N-(3-azanylpropyl)-3-[[(3S)-1-(2-fluorophenyl)-2-oxidanylidene-pyrrolidin-3-yl]amino]-N-methyl-benzamide 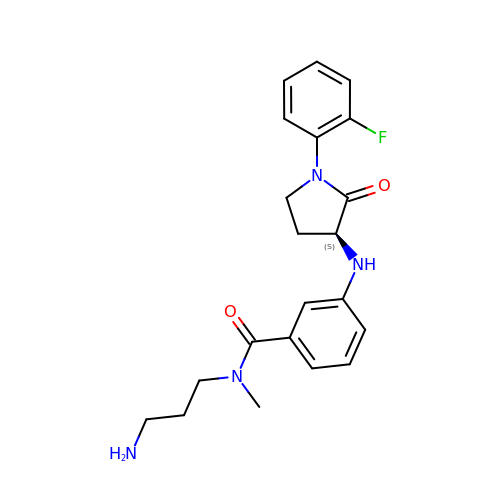| C21 H25 F N4 O2 | FKBZAUSZYONVAZ-SFHVURJKSA-N>[2x]MNSTPKGTIYLTFSDGPVNASVEVIKVLNQGGVKATFYFNAWHLDGIGDENEDRALEALKLALDSGHIVGNHSYDHMIHNCVEEFGPTSGADCNATGNHQIHSYQDPVRDAASFEQNLITLEKYLPTIRSYPNYKGYELARLPYTNGWRVTKHFQADGLCA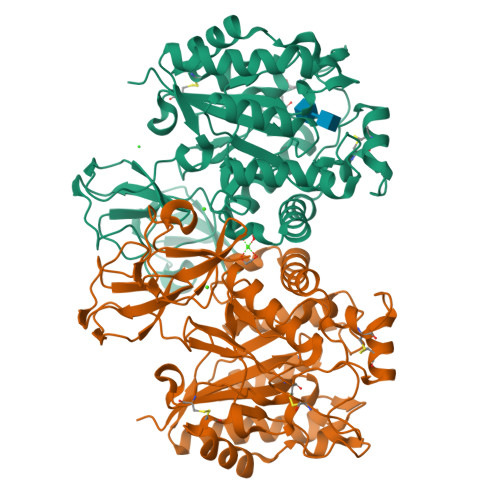TSDNLKPWEPGYVCDPANPSNSVKASIQVQNILANQGYQTHGWDVDWAPENWGIPMPANSLTEAVPFLAYVDKALNSCSPTTIEPINSKTQEFPCGTPLHADKVIVLTHDFLFEDGKRGMGATQNLPKLAEFIRIAKEAGYVFDTMDNYTPRWSVGKTYQAGEYVLYQGVVYKAVISHTAQQDWAPSSTSSLWTNADPATNWTLNVSYEQGDIVNYKGKRYLVSVPHVSQQDWTPDTQNTLFTALELRRQWSHPQFEK> MHHHHHHGSEEQEKALNFGIIS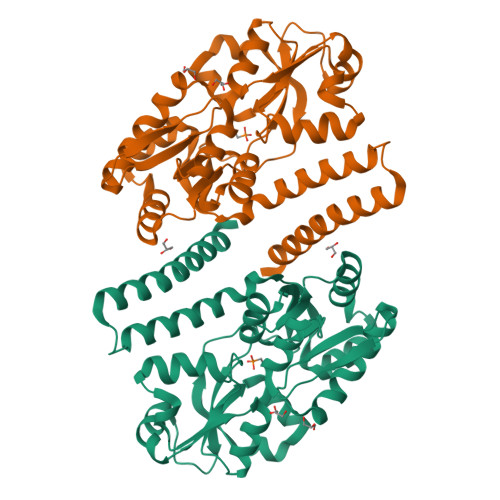TESQQNLKPQWTPFLQDMEKKLGVKVNAFFAPDYAGIIQGMRFNKVDIAWYGNLSAMEAVDRANGQVFAQTVAADGSPGYWSVLIVNKDSPINNLNDLLAKRKDLTFGNGDPNSTSGFLVPGYYVFAKNNISASDFKRTVNAGHETNALAVANKQVDVATNNTENLDKLKTSAPEKLKELKVIWKSPLIPGDPIVWRKNLSETTKDKIYDFFMNYGKTPEEKAVLERLGWAPFRASSDLQLVPIRQLALFKEMQSVKDNKGLNEQDKLAKTTAIQAQLDDLDRLNNALSAMSSVSKAVQ>[4x]MKYVVVSGGVISGIGKGVLASSTGMLLKTLGLKVTSIKIDPYMNIDAGTMSPLEHGECFVLDDGGETDLDLGNYERYLGITLSRDHNITTGKIYSHVISRERRGDYLGKTVQIVPHLTNAIQDWIQRVSKIPVDDTGLEPDVCIIELGGTVGDIESAPFVEALRQFQFEVGRENFALIHVSLVPVIHGEQKTKPTQAAIKDLRSLGLIPDMIACRCSEELNRSTIDKIAMFCHVGPEQVVNVHDVNSTYHVPLLLLKQHMIDYLHSRLKLGEVPLTLEDKERGSQLLTNWENMTKNLDDSDDVVKIALVGKYTNLKDSYLSVTKSLEHASMKCRRQLEILWVEASNLEPETQEVDKNKFHDSWNKLSSADGILVPGGFGTRGIEGMILAAKWARESGVPFLGVCLGLQVAAIEFARNVIGRPNSSSTEFLDETLLAPEDQVVITMRLGLRPTIFQPNSEWSNIRKLYGEVNEVHERHRHRYEINPKIVNDMESRGFIFVGKDETGQRCEIFELKGHPYYVGTQYHPEYTSKVLEPSRPFWGLVAAASGTLGEVIKDINL

CTP synthase (CTPS) catalyzes the final, rate-limiting step of de novo CTP biosynthesis (Lieberman, 1956). Each CTPS monomer consists of a glutaminase domain and an amido-ligase domain connected by an alpha helical linker. Glutamine hydrolysis in the glutaminase domain produces ammonia which is transferred through a channel into the amido-ligase domain, where it is ligated to UTP to form CTP in an ATP-dependent process. Budding yeast have two CTPS isoforms, Ura7 and Ura8, which share 78 % identical residues.

The Ura8 product-bound filament is in the canonical inhibited conformation, but the substrate-bound structure is in a conformation intermediate between canonical active and inhibited states, in which the ammonia channel remains closed. This suggested to us that one function of yeast CTPS filaments is to constrain the enzyme in a low activity conformation. To test this hypothesis, we determined the structure of free Ura8 tetramers at pH 7.4 bound to substrates at 2.8 Å resolution. In this unassembled state, Ura8 adopts the canonical active conformation, very similar to hCTPS2, including opening of the ammonia channel and rearrangement at the tetramerization interface. The active state we observe in free tetramers is incompatible with filament assembly, because in this conformation filament interfaces cannot be occupied on both sides of the tetramer simultaneously. Thus, filament assembly with symmetric contacts acts as a steric constraint to trap yeast CTPS in a low activity conformation, while tethering through a single glutaminase domain supports short, flexible filaments that accommodate a fully active conformation.>LNNVVIVGGGTAGWMTASYLKAAFGDRIDITLV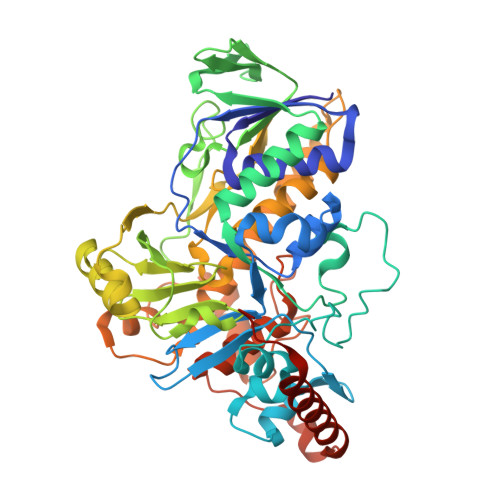ESGHIGAVGVGEATFSDIRHFFEFLGLKEKDWMPACNATYKLAVRFENWREKGHYFYHPFEQMRSVNGFPLTDWWLKQGPTDRFDKDCFVMASVIDAGLSPRHQDGTLIDQPFDEGADEMQGLTMSEHQGKTQFPYAYQFEAALLAKYLTKYSVERGVKHIVDDVREVSLDDRGWITGVRTGEHGDLTGDLFIDCTGFRGLLLNQALEEPFISYQDTLPNDSAVALQVPMDMERRGILPCTTATAQDAGWIWTIPLTGRVGTGYVYAKDYLSPEEAERTLREFVGPAAADVEANHIRMRIGRSRNSWVKNCVAIGLSSGFVEPLESTGIFFIHHAIEQLVKNFPAADWNSMHRDLYNSAVSHVMDGVREFLVLHYVAAKRNDTQYWRDTKTRKIPDSLAERIEKWKVQLPDSETVYPYYHGLPPYSYMCILLGMGGIELKPSPALALADGGAAQREFEQIRNKTQRLTEVLPKAYDYFTQ[2x]> MKLYVFLVNTGTTLTFDTELTVQTVADLKHAIQSKYKIAIQHQVLVVNGGECMAADRRVCTYSAGTDTNPIFLFNKEMILCDRPPAIPKTTFSTENDMEIKVEESLMMPAVFHTVASRTQLALEMYEVAKKLCSFCEGLVHDEHLQHQGWAA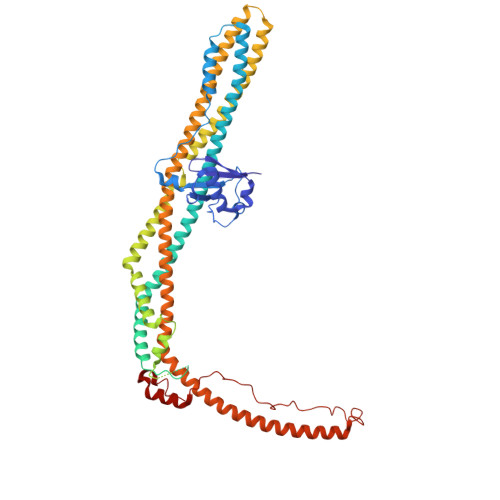IMANLEDCSNSYQKLLFKFESIYSNYLQSIEDIKLKLTHLGTAVSVMAKIPLLECLTRHSYRECLGRLDSLPEHEDSEKAEMKRSTELVLSPDMPRTTNESLLTSFPKSVEHVSPDTADAESGKEIRESCQSTVHQQDETTIDTKDGDLPFFNVSLLDWINVQDRPNDVESLVRKCFDSMSRLDPRIIRPFIAECRQTIAKLDNQNMKAIKGLEDRLYALDQMIASCGRLVNEQKELAQGFLANQKRAENLKDASVLPDLCLSHANQLMIMLQNHRKLLDIKQKCTTAKQELANNLHVRLKWCCFVMLHADQDGEKLQALLRLVIELLERVKIVEALSTVPQMYCLAVVEVVRRKMFIKHYREWAGALVKDGKRLYEAEKSKRESFGKLFRKSFLRNRLFRGLDSWPPSFCTQKPRKFDCELPDISLKDLQFLQSFCPSEVQPFLRVP> GETGQVIKSAVRSTVENTVQSTHSITTEATPALQAAETGATSNASDESMIETRNVVNTHGVAETSLEAFYGRAGLVAMFSTDGGIYRWYINFGEYVQLRAKLELLTYARFDMEFTIVAQVVNAQSKVQDFNVDYQVMFVPPGASVPENQDSYQWQSSCNPSVISNTGLPPARVSVPFMSSANAYSFSYDGYTQFGDTSGSSYGIVPSNYLGMLVVRTCEDLDGTRLRVRVYAKPKHVKGWIPRSPRMTPYKSRYTGVYTDTTKFCANRARIT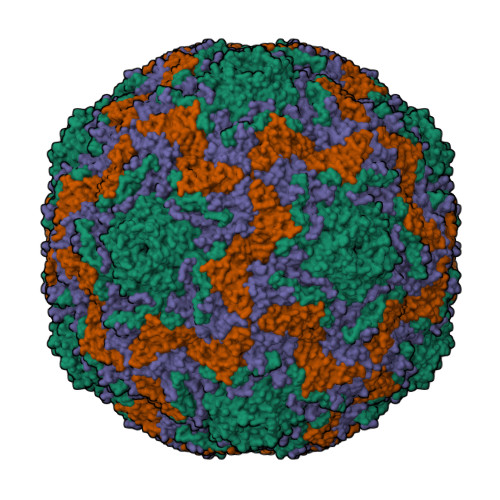TAG;> SAEACGYSDRVAQLTLGNSTITTQEAANIVVGYGRWPTSLRDTDATAVDKPTQPGVSAERFYTLPSVQWTNSFKGHYWKLPDALSELGLFGQNLQFHYLYRGGWVIHVQCNATKFHQGTLLVVATPEHKIQSAESPAFARTNPGEQGAAYQFPFTFEDGTALGNALIYPHQWVNLRTNNSATLVLPYVNALPMDSGIRHNNWTLSVIPIVPLEYAAGATTYVPITVTIAPMCTEYNGLRAAVTQ;> GIPTLYTPGSGQFLTTDDFQTPCMLPKFQPTPVIDIPGEVKNFLEVVQVESLVEINNVESAEGVARYRIPLNVQDAMDGQIMALRVDPGIDGPMQSTLLGVFTRYYAQWSGSLDFTFMFCGTFMTTGKVIIAYTPPGGDQPTNRRQAMLGTHVVWDFGLQSSITLVVPWISSGHFRGTTLENTIYKYRYYEAGYITMWYQTNMVVPPNFPTTASILMFVAAQPNFSLRILKDRPDISQEGALQ;> MGAQMSKNTAGSHTTGTYATGGSNIHYTNINYYENAASNSLNKQDFTQDPEKFTRPVVDVMKEAAVPLKSP>GMHIQPGLCGLGNLGNTCFMNSALQCLSNTAPLTDYFLKDEYEAEINRDNPLGMKGEIAEAYAELIKQMWSGRDAHVAPRMFKTQVGRFAPQFSGYQQQDSQELLAFLLDGLHEDLNRVKKKPYLELKDANGRPDAVVAKEAWENHRLRNDSVIVDTFHGLFKSTLVCPECAKVSVTFDPFCYLTLPLPLKKDRVMEGPMLQPQKKKKTTVALRDCIELFTTMETLGEHDPWYCPNCKKHQQATKKFDLWSLPKILVVHLKRFSYNRYWRDKLDTVVEFPIRGLNMSEFVCNLSARPYVYDLIAVSNHYGAMGVGHYTAYAKNKLNGKWYYFDDSNVSLASEDQIVTKAAYVLFYQRRDDEFYKTPS[6x]

USP4 is involved in different cellular pathways and targets a variety of substrates. USP4 features a large domain (~30 kDa, named USP4 insert from here on) inserted within the catalytic core, which carries a Ubl domain. A tandem DUSP–Ubl domain2526 is located at the N-terminus of the protein and is separated from the catalytic domain by a connecting linker. In this study we show that USP4 requires the N-terminal DUSP–Ubl domain to achieve its full catalytic turnover in vitro.

On the basis of a multi-sequence alignment of USP family members, we concluded that the protease treatment removed an insertion between L481 and L766 (USP4 insert). The two fragments were coexpressed and purified yielding a minimal catalytic domain (USP4 D1D2). The structure was refined to 2.4 Å resolution with an R/Rfree of 0.178/0.21 and good geometry. There are six molecules of USP4 D1D2 per asymmetric unit with equivalent conformation (root mean squared deviation of 0.7 Å over 344 Cαs, calculated with SSM software). The fold of USP4 D1D2 is similar to that of other USP catalytic domains, resembling an extended right hand comprising three domains: fingers, thumb and palm. The D1 fragment contains the thumb domain and part of the fingers domain including the USP signature conserved sequences ‘Cys box’ and ‘QQD box’ of the active site, whereas the D2 fragment completes the active site with the ‘His box’ and the rest of the fingers and palm domains. In the finger domain, D1 and D2 are brought together by a Zn2+ ion coordinated by cysteine residues belonging to both domains. This zinc-finger ribbon (observed also in USP2, USP8 and USP21 structures) is in the contracted ‘closed-hand' configuration seen in USP8, which was proposed to block ubiquitin access. Superposition of the six non-crystallographic symmetry-related molecules of USP4 D1D2 shows flexibility in the zinc-finger ribbon (maximal Cα displacement 4 Å), suggesting that it can move to accommodate ubiquitin. In USP4 the position of BL1, BL2 and SL hinders the access of ubiquitin to the catalytic domain, suggesting that the flexibility observed in these loops is required for the dynamic exchange of ubiquitin in and out of the active site.> GSHMSRKIRDLIESKRFQNVITAIIVLNGAVLGLLTDTTLSASSQNLLERVD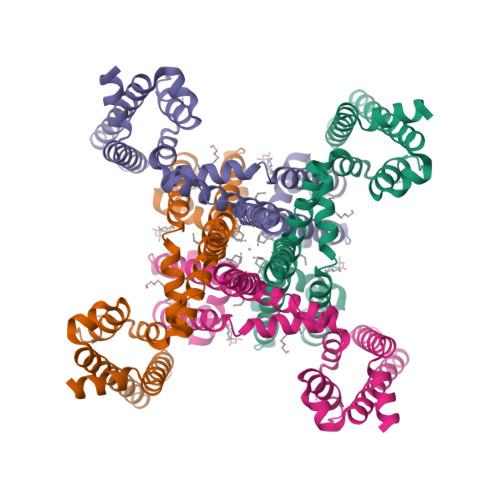QLCLTIFIVEISLKIYAYGVRGFFRSGWNLFDFVIVAIALMPAQGSLSVLRTFRIFRVMRLVSVIPTMRRVVQGMLLALPGVGSVAALLTVVFYIAAVMATNLYGATFPEWFGDLSKSLYTLFQVMTLESWSMGIVRPVMNVHPNAWVFFIPFIMLTTLTVLNLFIGIIVDAMAITKEQEEEAKTGHHQEPISQTLLHLGDRLDRIEKQLAQNNELLQRQQPQKK>[3x]MGEGPELHLASQFVNEACRALVFGGCVEKSSVSRNPEVPFESSAYRISASARGKELRLILSPLPGAQPQQEPLALVFRFGMSGSFQLVPREELPRHAHLRFYTAPPGPRLALCFVDIRRFGRWDLGGKWQPGRGPCVLQEYQQFREN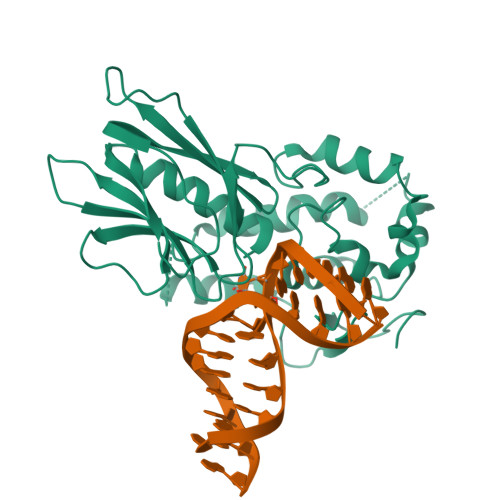VLRNLADKAFDRPICEALLDQRFFNGIGNYLRAEILYRLKIPPFEKARSVLEALQQHRPSPELTLSQKIRTKLQNPDLLELCHSVPKEVVQLGGRGYGSESGEEDFAAFRAWLRCYGMPGMSSLQDRHGRTIWFQGDPGPLAPKGRKSRKKKSKATQLSPEDRVEDALPPSKAPSRTRRAKRDLPKRTATQRPEGTSLQQDPEAPTVPKKGRRKGRQAASGHCRPRKVKADIPSLEPEGTSASAALGHHHHHH> MEKSVSVILLAGGQGKRMKMSMPKQYIPLLGQPIALYSFFTFSRMPEVKEIVVVCDPFFRDIFEEYEESIDVDLSFAIPGKERQ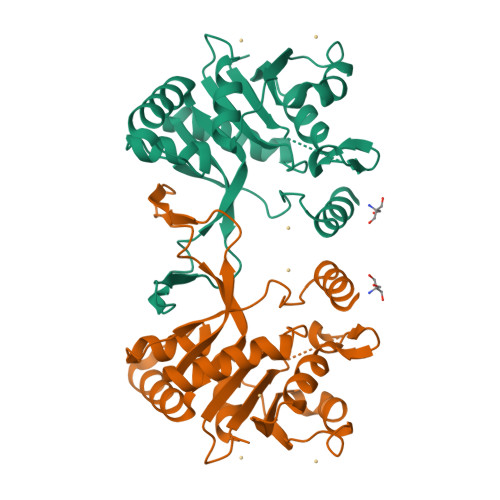DSVYSGLQEIDVNSELVCIHDSARPLVNTEDVEKVLKDGSAVGAAVLGVPAKATIKEVNSDSLVVKTLDRKTLWEMQTPQVIKPELLKKGFELVKSEGLEVTDAVSIVEYLKHPVYVSQGSYTNIKVTTPDDLLLAERILSEDS>MKLFLILLVLPLASCFFTCNSNANLSMLQLGVPDNSSTIVTGLLPTHWFCANQSTSVYSANGFFYIDVGNHRSAFALHTGYYDANQYYIYVTNEIGLNASVTLKICKFSRNTTFDFLSNASSSFDCIVNLLFTEQLGAPLGITISGETVRLHLYNVTRTFYVPAAYKLTKLSVKCYFNYSCVFSVVNATVTVNVTTHNGRVVNYTVCDDCNGYTDNIFSVQQDGRIPNGFPFNNWFLLTNGSTLVDGVSRLYQPLRLTCLWPVPGLKSSTGFVYFNATGSDVNCNGYQHNSVVDVMRYNLNFSANSLDNLKSGVIVFKTLQYDVLFYCSNSSSGVLDTTIPFGPSSQPYYCFINSTINTTHVSTFVGILPPTVRE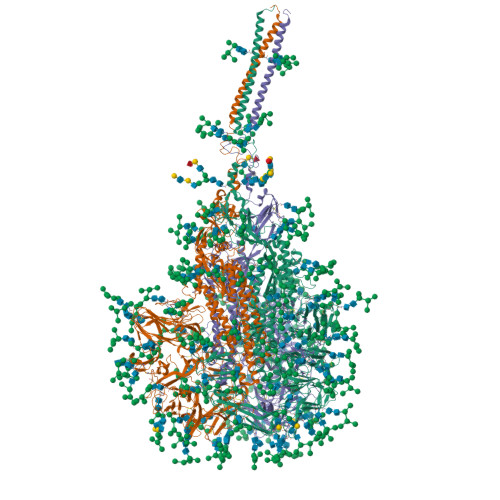IVVARTGQFYINGFKYFDLGFIEAVNFNVTTASATDFWTVAFATFVDVLVNVSATNIQNLLYCDSPFEKLQCEHLQFGLQDGFYSANFLDDNVLPETYVALPIYYQHTDINFTATASFGGSCYVCKPHQVNISLNGNTSVCVRTSHFSIRYIYNRVKSGSPGDSSWHIYLKSGTCPFSFSKLNNFQKFKTICFSTVEVPGSCNFPLEATWHYTSYTIVGALYVTWSEGNSITGVPYPVSGIREFSNLVLNNCTKYNIYDYVGTGIIRSSNQSLAGGITYVSNSGNLLGFKNVSTGNIFIVTPCNQPDQVAVYQQSIIGAMTAVNESRYGLQNLLQLPNFYYVSNGGNNCTTAVMTYSNFGICADGSLIPVRPRNSSDNGISAIITANLSIPSNWTTSVQVEYLQITSTPIVVDCATYVCNGNPRCKNLLKQYTSACKTIEDALRLSAHLETNDVSSMLTFDSNAFSLANVTSFGDYNLSSVLPQRNIRSSRIAGRSALEDLLFSKVVTSGLGTVDVDYKSCTKGLSIADLACAQYYNGIMVLPGVADAERMAMYTGSLIGGMVLGGLTSAAAIPFSLALQARLNYVALQTDVLQENQKILAASFNKAINNIVASFSSVNDAITQTAEAIHTVTIALNKIQDVVNQQGSALNHLTSQLRHNFQAISNSIQAIYDRLDSIQADQQVDRLITGRLAALNAFVSQVLNKYTEVRGSRRLAQQKINECVKSQSNRYGFCGNGTHIFSIVNSAPDGLLFLHTVLLPTDYKNVKAWSGICVDGIYGYVLRQPNLVLYSDNGVFRVTSRVMFQPRLPVLSDFVQIYNCNVTFVNISRVELHTVIPDYVDVNKTLQEFAQNLPKYVKPNFDLTPFNLTYLNLSSELKQLEAKTASLFQTTVELQGLIDQINSTYVDLKLLNRFENYIKWPWWVWLIISVVFVVLLSLLVFCCLSTGCCGCCNCLTSSMRGCCDCGSTKLPYYEFEKVHVQ[3x]> MVEFSLKKARNNWKHVKKSASSPAKQKTPPSPAKPKQKTKKNPYSDLKDPATSYTLPTINARERSRVATSMQRRLSIHNTNYAPPTLDYSMPLPDMPNMIVPNDNVDSSHNNSSFTTENESVSSKGPSNSLNLSTADLSLNDSSYNKVPARSAMRNTVNPSGSNDPFNNSTSLRKMLANPHFNAKDFVHDKLGNASAITIDKFTSNLTDLSIQVQEEVKLNINKSYNEIMTVNNDLNVAMLELKRVRANINDLNEVLDQCTKIAEKRLQLQDQIDQERQGNFNNVESHSNSPALLPPLKAGQNGNLMRRDRSSVLILEKFWDTELDQLFKNVEGAQKFINSTKGRHILMNSANWMELNTTTGKPLQMVQIFILNDLVLIADKSRDKQNDFIVSQCYPLKDVTVTQEEFSTKRLLFKFSNSNSSLYECRDADECSRLLDVIRKAKDDLCDIFHVEEENSKRIRESFRYLQSTQQ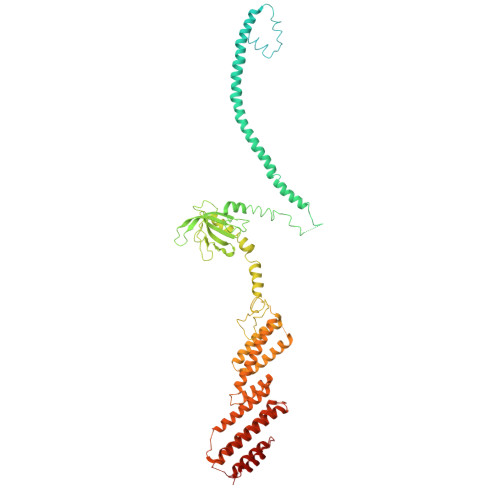TPGRENNRSPNKNKRRSMGGSITPGRNVTGAMDQYLLQNLTLSMHSRPRSRDMSSTAQRLKFLDEGVEEIDIELARLRFESAVETLLDIESQLEDLSERISDEELMLLNLISLKIEQRREAISSKLSQSILSSNEIVHLKSGTENMIKLGLPEQALDLFLQNRSNFIQDLILQIGSVDNPTNYLTQLAVIRFQTIKKTVEDFQDIFKELGAKISSILVDWCSDEVDNHFKLIDKQLLNDEMLSPGSIKSSRKQIDGLKAVGLDFVYKLDEFIKKNSDKIR>GPKHERFIAYVGIPMLTIQARENDDQIILGSLGSQRMKYIEDENQNYTNISSEYYSQSSMQAVPMYYFNVPKGQWSVDISCEGYQPTSSTSDPHRGRSDGMIAYSNADSDYWNVGEADGVKISKLRNDNTYRQGHPELEINSCHFREGQLLERDATISFHVEAPTDGRFFLVGPAIQKTAKYNYTISYGDWTDRDMELGL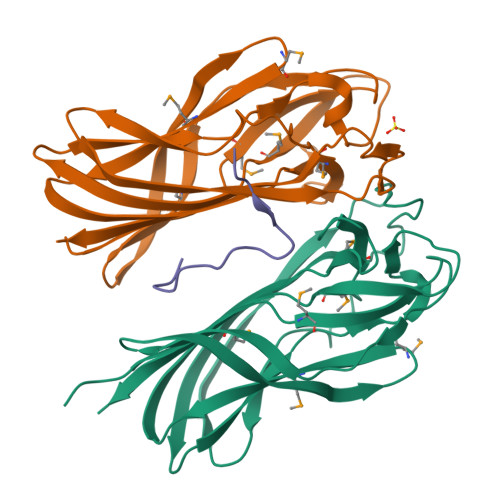ITVVLDEHL[2x];> EGTGSANRVRRPPREGHIYMAS> GPMIDLYTAATPNGHKVSIALEEMGLPYTVHALSFDKKEQKAPEFLRINPNG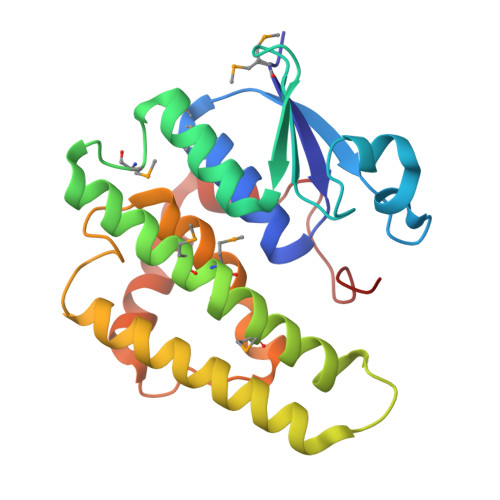RIPAIVDRSNDDFAVFESGAILVYLAEKTGQLMPTDVKGRSRVIQWLMFQMGGVGPMQGQANVFFRYFPEKLQGAIDRYQHETRRLYEVLDGRLGEAEYLAGDYSIADIATYPWVRIHDWSGVAVDGLDNLQRWIAALEARPAVQRGLLVPRREKEGDDAI>MDPSQTPDANASISVSYKCGVKDGTKNTIRATINIKNTGTTPVNLSDIKVRYWFTSDGNEQNNFVCDYAAFGTDKVKGIVKKIENS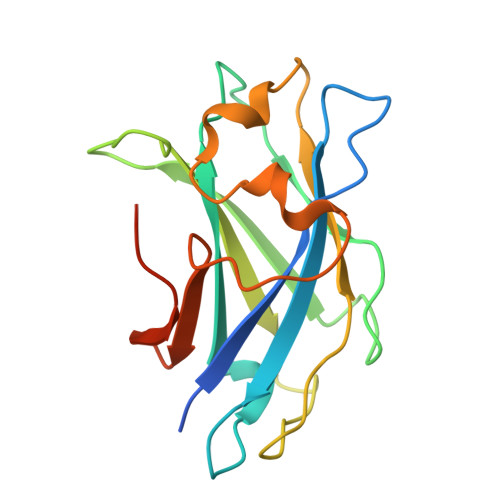VPGADTYCEISFTEDAGRLAPGGSTGTIPFRIEGAAEYDQTDDYSYNSEMSDDFGDNTKITAYIKDKLKYGVEAAALEHHHHHH[3x]>MSSRIRINTKSLLVQPGYSGSKMRDRLFFLLSKYGIRPRDSIGQHFLIIEDVIEKAIETANVNENDVILEVGPGLGFLTDELAKRAKKVYTIEIDQKIIEILKKEYSWNNVK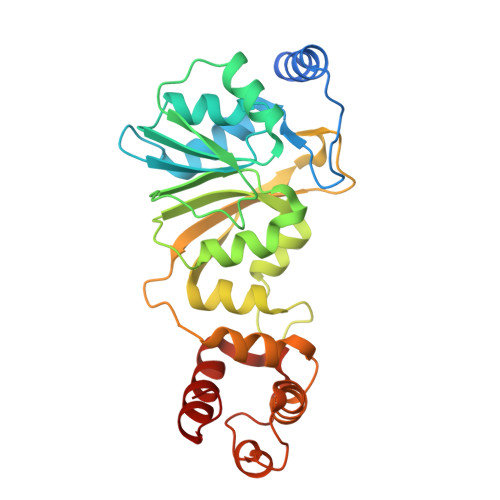IIQGAAVRVEWPKFNKVVSNIPYKISSPFTFKLLKTDFERAVVMYQLEFALRMVAKPGSRNYSRLSLMAQALGNVEIVMKIGKGAFYPRPKVDSALVLIEPRKDKIVLNENLVKALFQHRRKTVPRALKDSIHMLGVSKDEIRGIINNVPHSNKRVFQLYPEEVKDIEEYLKKHGIIS[2x]>MKLIVAIVRPEKLNEVLKALFQAEVRGLTLSRVQGHGGETERVETYRGTTVKMELHEKVRLEIGVSEPFVKPTVE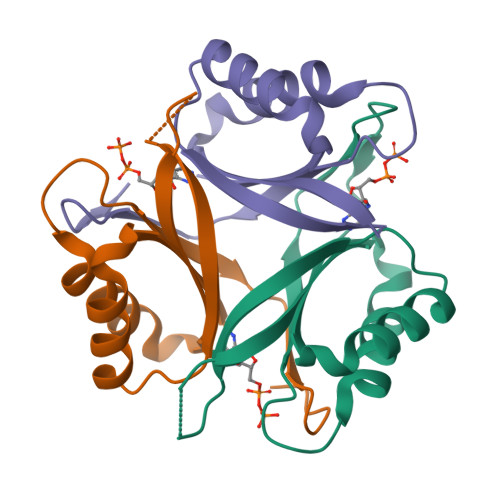AILKAARTGEVGDGKIFVLPVEKVYRIRTGEEDEAAVTPVQ[3x]>STTGIIMENVTAFWEEGFGELLEKVQQSNGDRKHSSDENNVSFSHLCLVGNPVLKNINLNIEKGEMLAITGSTGSGKTSLLMLILGELEASEGIIKHSGRVSFCSQF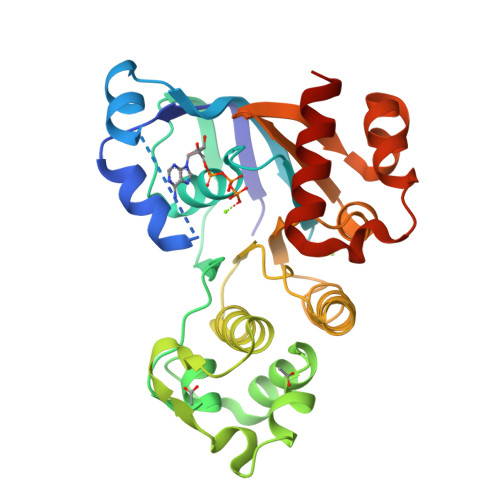SWIMPGTIKENIIGVSYDEYRYKSVVKACQLQQDITKFAEQDNTVLGEGGVTLSGGQRARISLARAVYKDADLYLLDSPFGYLDVFTEEQVFESCVCKLMANKTRILVTSKMEHLRKADKILILHQGSSYFYGTFSELQSLRPDFSSKLMGYDTFDQFTEERRSSILTETLRRFSVDD[4x]> GGAUCUUACUUGGUAGACUCGCAGGAAGUCUACCGAGUAAGAGAAAGAGGAAAGACGGCCAAAUUGCGGGAAAGGGGACAACAGCCGUUCAGUACCAAGUCUCAGGGAAACUUCAGAUGGCCUCGCAAAGGGUAUGGUAAUAAGCUGACGGACAUGGUCCUAACCACGCAGUCAAGUCCUAAGUCAACAGCCUUGGCUGUUGAUAUGGAUGCAUUUCGAUCCAACCGAGGCUCAUUCUUGUAAUUCAUGGCCGUCGGGGAGGCACUUCGGUGCCUCUG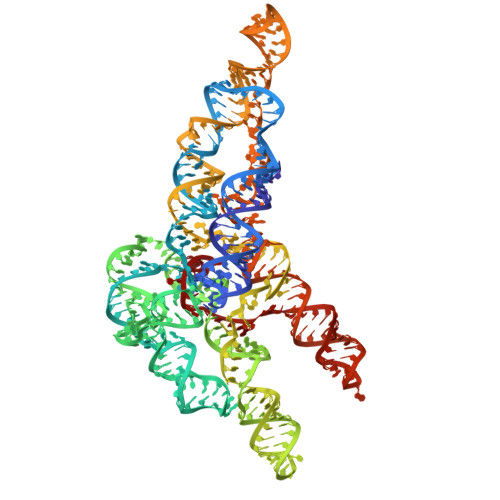AUAACAACUUGAAAUAAGGUUGGCUCAACGGCGCGUGACAGACAAUUCGCGCUGGAACUGCAGUCGGACCU[(7R)-4-(5-chloro-1,3-benzoxazol-2-yl)-7-methyl-1,4-diazepan-1-yl][5-methyl-2-(2H-1,2,3-triazol-2-yl)phenyl]methanone 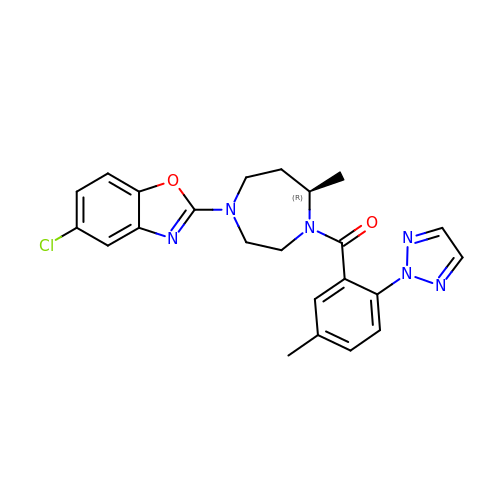| C23 H23 Cl N6 O2 | JYTNQNCOQXFQPK-MRXNPFEDSA-N>GSHMAAELDSLLGQEKERFQVLPGRDKMLYVAAQNERDTLWARQVLARGDYDKNARVINENEENKRISIWLDTYYPQLAYYRIHFDEPRKPVFWLSRQRNTMSKKELEVLSQKLRALMPYADSVNITLMDDVTAAGQAEAGLKQQALPYSRRNHKGGVTFVIQGALDDVEILRARQFVDSYYRTWGGRYVQF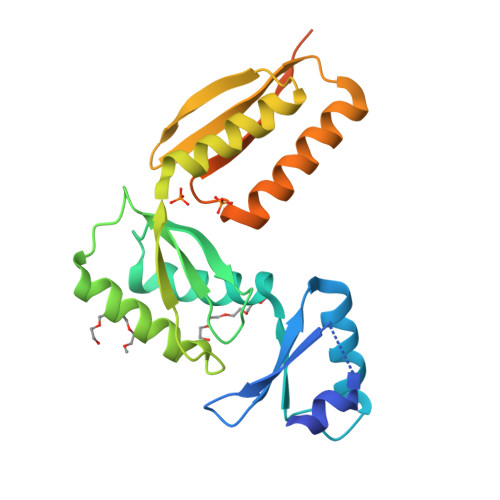AIELKDDWLKGRSFQYGAEGYIKMSPGHWYFPSPL[2x]1-deoxy-1-[(4aS)-4a-hydroxy-7,8-dimethyl-2,4-dioxo-3,4,4a,5-tetrahydrobenzo[g]pteridin-10(2H)-yl]-5-O-phosphono-D-ribitol | C17 H23 N4 O10 P | 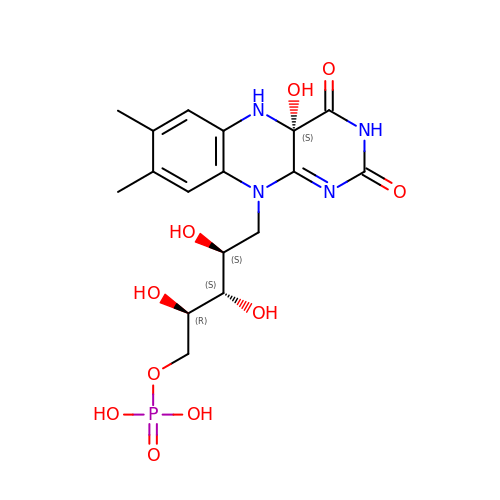XVRDTKNEVFQDDQ-LKQDWFRTSA-N>MLSKDIIKLLNEQVNKEMNSSNLYMSMSSWCYTGSRQGSLSGGNVSSSYSLDGCGTFLFDHAAEEYEHAKKLIVFLNENNVPVQLTSISAPEHKFEGLTQIFQKAYEHEQHISESINNIVDHAIKSKDHATFNFLQWYVSEQHEEEVLFKDILDKIELIGNENHG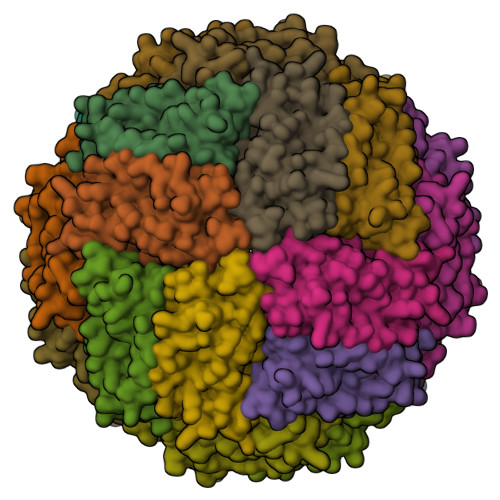LYLADQYVKGIAKSRKS[12x]Nalpha-[(benzyloxy)carbonyl]-N-[(2S)-1-phenyl-4-(phenylsulfonyl)butan-2-yl]-L-phenylalaninamide 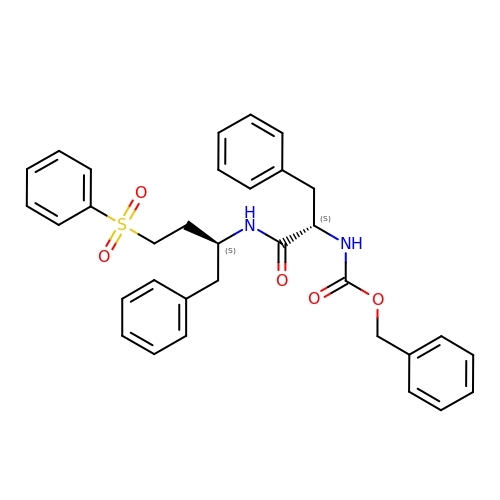| C33 H34 N2 O5 S | RLNXSKBHINXQAP-VEEOACQBSA-N> HLPKPTLWAEPGSVITQGSPVTLRCQGGQETQEYRLY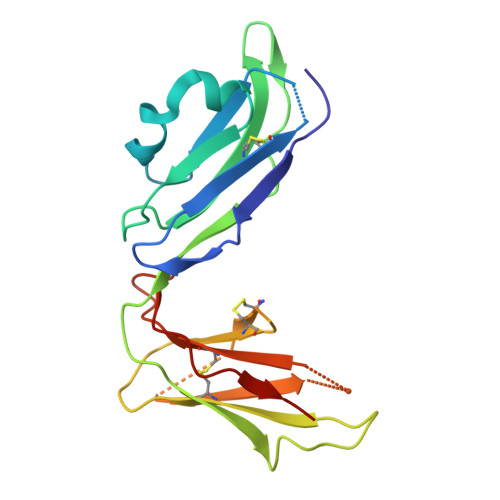REKKTAPWITRIPQELVKKGQFPIPSITWEHAGRYRCYYGSDTAGRSESSDPLELVVTGAYIKPTLSAQPSPVVNSGGNVTLQCDSQVAFDGFILCKEGEDEHPQCLNSQPHARGSSRAIFSVGPVSPSRRWWYRCYAYDSNSPYEWSLPSDLLELLVLG>[2x]SLAEIRTDFNILYSMMKKHEEFRWMRLRIRRMADAWIQAIKSLAEKQNLEKRKRKKVLVHLGLLTKESGFKIAETAFSGGPLGELVQWSDLITSLYLLGHDIRISASLAELKEIMKKVVGNRSGCPTVGDRIVELIYIDIVGLAQFKKTLGPSWVHYQCMLRVLDSFGTEPEFNHANYAQSKGHKTPWGKWNLNPQQFYTMFPHTPDNSFLGFVVEQHLNSSDIHHINEIKRQNQSLVYGKVDSFWKNKKIYLDIIHTYMEVHATVYGSSTKNIPSYVKNHGILSGRDLQFLLRETKLFVGLGFPYEGPAPLEAIANGCAFLNPKFNPPKSSKNTDFFIGKPTLRELTSQHPYAEVFIGRPHVWTVDLNNQEEVEDAVKAILNQKIEPYMPYEFTCEGMLQRINAFIEKQDFCHGQVMWPPLSALQVKLAEPGQSCKQVCQESQLICEPSFFQHLNKDKDMLKYKVTCQSSELAK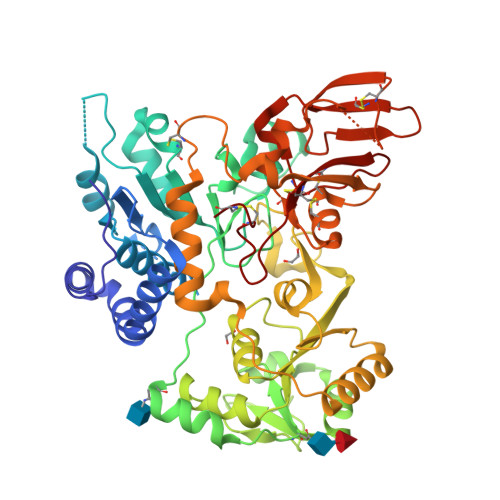DILVPSFDPKNKHCVFQGDLLLFSCAGAHPRHQRVCPCRDFIKGQVALCKDCL> MDEIISELRELCLNYIEQDERLSRQKLNFLGQREPRMVLIEGLKLLSRCIEIDSADKSGCTHNHDDKSVETILVESGIVCPGLPLIIPDGYKLIDNSLILLECFVRSTPASFEKKFIEDTNKLACIREDLAVAGVTLVPIVDGRCDYDNSFMPEWANFKFRDLLFKLLEYSNQNEKVFEESEYFRLCESLKTTIDKRSGMDSMKILKDARSTHNDEIMRMCHEGINPNMSCDDVVFGINSLFSRFRRDLESGKLKRNFQKVNPEGLIKEFSELYENLADSDDILTLSREAVESCPLMRFITAETHGHERGSETSTEYERLLSMLNKVKSLKLLNTRRRQLLNLDVLCLSSLIKQSKFKGLKNDKHWVGCCYSSVNDRLVSFHSTKEEFIRLLRNRKKSKVFRKVSFEELFRASISEFIAKIQKCLLVVGLSFEHYGLSEHLEQECHIPFTEFENFMKIGAHPIMYYTKFEDYNFQPSTEQLKNIQSLRRLSSVCLALTNSMKTSSVARLRQNQIGSVRYQVVECKEVFCQVIKLDSEEYHLLYQKTGESSRCYSIQGPDGHLISFYADPKRFFLPIFSDEVLYNMIDIMISWIRSCPDLKDCLTDIEVALRTLLLLMLTNPTKRNQKQVQSVRYLVMAIVSDFSSTSLMDKLREDLITPAEKVVYKLLRFLIKTIFGTGEKVLLSAKFKFMLNVSYLCHLITKETPDRLTDQIKCFEKFFEPKSQFGFFVNPKEAITPEEECVFYEQMKRFTSKEIDCQHTTPGVNLEAFSLMVSSFNNGTLIFKGEKKLNSLDPMTNSGCATALDLASNKSVVVNKHLNGERLLEYDFNKLLVSAVSQITESFVRKQKYKLSHSDYEYKVSKLVSRLVIGSKGEETGRSEDNLAEICFDGEEETSFFKSLEEKVNTTIARYRRGRRANDKGDGEKLTNTKGLHHLQLILTGKMAHLRKVILSEISFHLVEDFDPSCLTNDDMKFICEAVEGSTELSPLYFTSVIKDQCGLDEMAKNLCRKFFSENDWFSCMKMILLQMNANAYSGKYRHMQRQGLNFKFDWDKLEEDVRISERESNSESLSKALSLTKCMSAALKNLCFYSEESPTSYTSVGPDSGRLKFALSYKEQVGGNRELYIGDLRTKMFTRLIEDYFESFSSFFSGSCLNNDKEFENAILSMTINVREGFLNYSMDHSKWGPMMCPFLFLMFLQNLKLGDDQYVRSGKDHVSTLLTWHMHKLVEVPFPVVNAMMKSYVKSKLKLLRGSETTVTERIFRQYFEMGIVPSHISSLIDMGQGILHNASDFYGLLSERFINYCIGVIFGERPEAYTSSDDQITLFDRRLSDLVVSDPEEVLVLLEFQSHLSGLLNKFISPKSVAGRFAAEFKSRFYVWGEEVPLLTKFVSAALHNVKCKEPHQLCETIDTIADQAIANGVPVSLVNSIQRRTLDLLKYANFPLDPFLLNTNTDVKDWLDGSRGYRIQRLIEELCPNETKVVRKLVRKLHHKLKNGEFNEEFFLDLFNRDKKEAILQLGDLLGLEEDLNQLADVNWLNLNEMFPLRMVLRQKVVYPSVMTFQEERIPSLIKTLQNKLCSKFTRGAQKLLSEAINKSAFQSCISSGFIGLCKTLGSRCVRNKNRENLYIKKLLEDLTTDDHVTRVCNRDGITLYICDKQSHPEAHRDHICLLRPLLWDYICISLSNSFELGVWVLAEPTKGKNNSENLTLKHLNPCDYVARKPESSRLLEDKVNLNQVIQSVRRLYPKIFEDQLLPFMSDMSSKNMRWSPRIKFLDLCVLIDINSESLSLISHVVKWKRDEHYTVLFSDLANSHQRSDSSLVDEFVVSTRDVCKNFLKQVYFESFVREFVATTRTLGNFSWFPHKEMMPSEDGAEALGPFQSFVSKVVNKNVERPMFRNDLQFGFGWFSYRMGDVVCNAAMLIRQGLTNPKAFKSLKDLWDYMLNYTKGVLEFSISVDFTHNQNNTDCLRKFSLIFLVRCQLQNPGVAELLSCSHLFKGEIDRRMLDECLHLLRTDSVFKVNDGVFDIRSEEFEDYMEDPLILGDSLELELLGSKRILDGIRSIDFERVGPEWEPVPLTVKMGALFEGRNLVQNIIVKLETKDMKVFLAGLEGYEKISDVLGNLFLHRFRTGEHLLGSEISVILQELCIDRSILLIPLSLLPDWFAFKDCRLCFSKSRSTLMYETVGGRFRLKGRSCDDWLGGSVAEDID;> MGQGKSREEKGTNSTNRAEILPDTTYLGPLSCKSCWQKFDSLVRCHDHYLCRHCLNLLLSVSDRCPLCKYPLPTRLKISTAPSSPPPYEE

Lymphocytic choriomeningitis virus (LCMV) is the prototypic member of the Arenaviridae family and belongs to the Old World (OW) arenavirus together with Lassa virus (LASV), which are distinct from the New World (NW) arenavirus [e.g. Machupo virus (MACV) and Junin virus (JUNV)]. As a segmented negative-sense single-stranded RNA virus (sNSRV), arenavirus encodes a large polymerase (L) to form a ribonucleoprotein complex (RNP) together with the genomic-length RNA encapsidated by viral nucleoprotein (NP) and facilitate virus replication and transcription. Arenavirus also encodes a RING finger Z matrix protein as a regulator of RNA synthesis. Previous studies have shown that the arenavirus Z protein forms a species-specific complex with the L protein and inhibits RNA synthesis initiation by impairing the catalytic activity of the L protein, which is known to be essential for the balance of infection and further initiation of virion assembly; however, the mechanism remains unclear.

In the LCMV L–Z complex structure, L and Z form a heterodimer with a molar ratio of 1:1. The final model of the LCMV L–Z complex includes residues 1–1814 of L and residues 28–74 of Z. The Z protein was found to bind at the bottom of the interface between the core lobe of the PA-like domain and the palm subdomain of the RdRp core. The position of Z partially blocks the product exit tunnel for the releasing nascent RNA product. Although the full-length Z was used to generate the L–Z complex, only its zinc finger domain can be built in the complex structure, suggesting that its N-/C-terminal portions are flexible and do not participate in the interaction with L. The zinc finger domain of LCMV-Z contains a single α-helix and two β-strands and harbors two zinc ions by residues C32–C35–C51–C54 and C45–H48–C65–C68 to form two zinc fingers, which are conserved with that observed in LASV-Z. The LCMV L–Z interaction comprises a set of hydrophobic interactions, hydrogen bonds, and van de Waals interactions with a large intermolecular contact surface of ~780 Å2, which is 20% of the ~4,000 Å2 total area of the molecular face of Z. The interacting residues of Z are located on the surface at the side of the two zinc-binding sites, including P29, S34, C35, W36, Q37, C54, L57, L58, V61, P66 and L67. Compared with apo LCMV-L, the core lobe, head lobe, and clamp domain of the PA-like region have a 1.7° orientation shifting apart from the RdRp core with the binding site of Z as the fixed point. With the binding of Z, only one α-helix can be observed, and most parts of the α-ribbon motif lack interpretable cryo-EM density, suggesting that these parts have a flexible architecture. Moreover, an additional conformational change of an α-helix in the palm subdomain can be observed in the LCMV L–Z complex.4-chloro-7-nitrobenzofurazan | C6 H2 Cl N3 O3 | 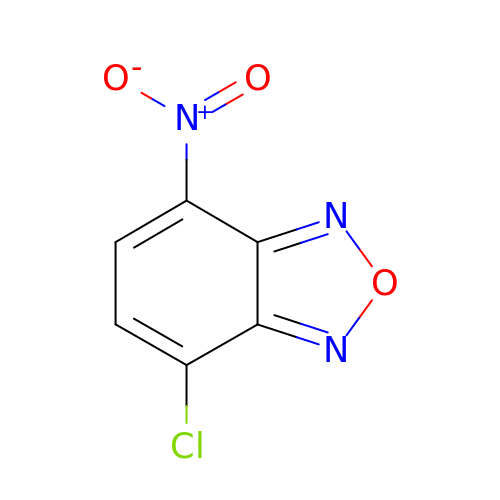IGHBXJSNZCFXNK-UHFFFAOYSA-N> GSHMSGIALSRL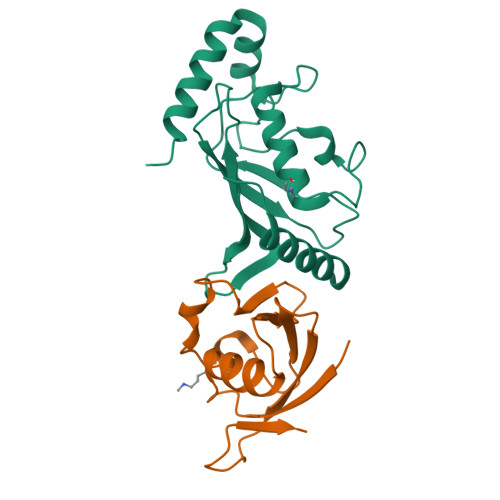AQERKAWRKDHPFGFVAVPTKNPDGTMNLMNWECAIPGKKGTPWEGGLFKLRMLFKDDYPSSPPKCKFEPPLFHPNVYPSGTVCLSILEEDKDWRPAITIKQILLGIQELLNEPNIQDPAQAEAYTIYCQNRVEYEKRVRAQAKKFAPS;> GSHSKPEVTVRLNVHKVTVLTLQDKIVKEKFAMVAPDVQIEDGKGTILISSEEGETEANNHKKLSEFGIRNGSRLQADDFLQDYTLLINILHSEDLGKDVEFEVV>YQLEKEPIVGAETFYVDGAANRETKLGKAGYVTNKGRQKVVPLTNTTNQKTELQAIYLALQDSGLEVN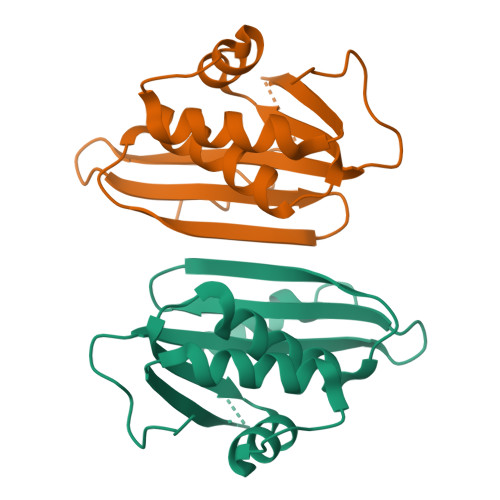IVTDSQYALGIIQAQPDKSESELVNQIIEQLIKKEKVYLAWVPAHKGIGGNEQVDKLVSAGIRKILFL[2x]> SMDFKENPNLRDNWTDAEGYYRVNIGEVLDKRYNVYGYTGQGVFSNVVRARDNARA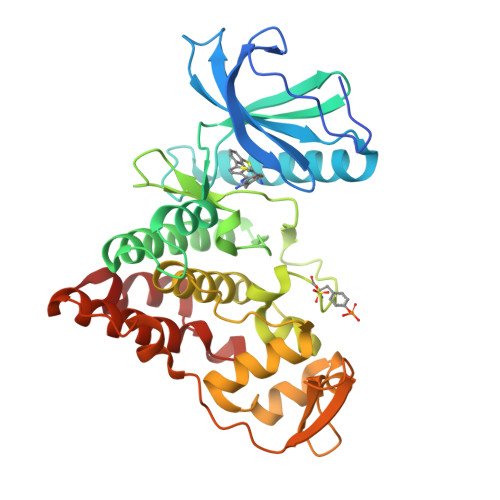NQEVAVKIIRNNELMQKTGLKELEFLKKLNDADPDDKFHCLRLFRHFYHKQHLCLVFEPLSMNLREVLKKYGKDVGLHIKAVRSYSQQLFLALKLLKRCNILHADIKPDNILVNESKTILKLCDFGSASHVADNDITPYLVSRFYRAPEIIIGKSYDYGIDMWSVGCTLYELYTGKILFPGKTNNHMLKLAMDLKGKMPNKMIRKGVFKDQHFDQNLNFMYIEVDKVTEREKVTVMSTINPTKDLLADLIGCQRLPEDQRKKVHQLKDLLDQILMLDPAKRISINQALQHAFIQE5-(HYDROXY-METHYL-AMINO)-3-METHYL-PYRROLIDINE-2-CARBOXYLIC 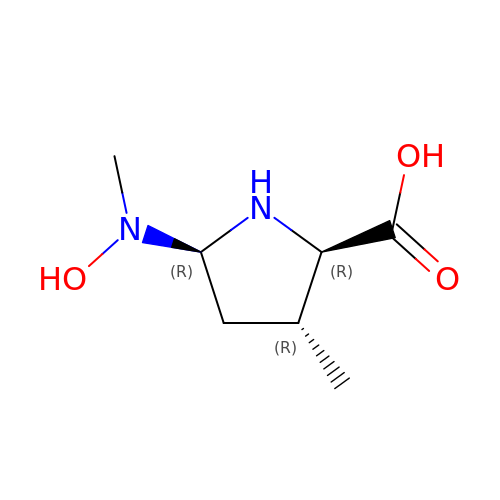ACID | C7 H14 N2 O3 | PGYJBAGGGAUHGV-HSUXUTPPSA-N> MTLGTNQVSKTHSFMTVSLIELWERFGYYGMQALIVYFMVQRLGFDDSRANLVWSACAALIYVSPAIGGWVGDKILGTKRTMLLGAGILSVGYALMTVPTENTWFMFSALGVIVVGNGLFKPNAGNLVRKIYEGDDSKIDSAFTIYYMAVNVGSTFSMLLTPWIKD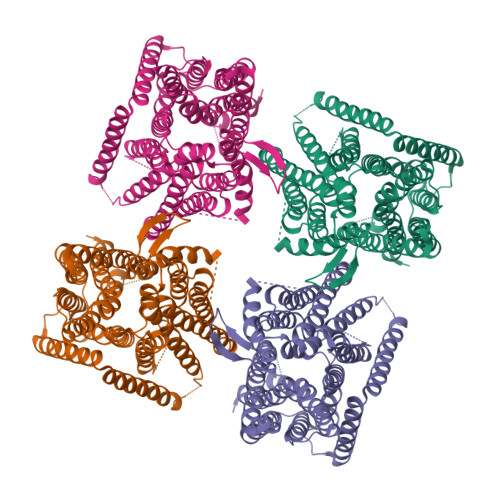YVNAQYGNEFGWHAAFAVCCVGILVGLGNYALMHKSLANYGSEPDTRPVNKKSLAIVLALAALSVVASAIILEYEDVARVFVYAAGVAVLGIFFHLIRTSEPSERAGLIAALILTVQTVFFFIFYQQMSTSLALFALRNVDWDFQVFGTHLWTWSPAQFQALNPIWIMVLSPVLAWSYSWAGRNNKDFSIAAKFALGFAVVAIGFFIYGFAGQFAVNGKTSSWVMIWGYASYSLGELLVSGLGLAMIARYVPARMGGFMMGAYFVASGISQYLGGVVANFASVPQDLVDPLQTLPVYTNLFNKLGVAAVVCTIIALAVLPLMRRLTESHHAHSSIENNAAASLRDVKAEQLESSGENLYFQ>[8x]AMWHTHSEREKRVSNAVEFLL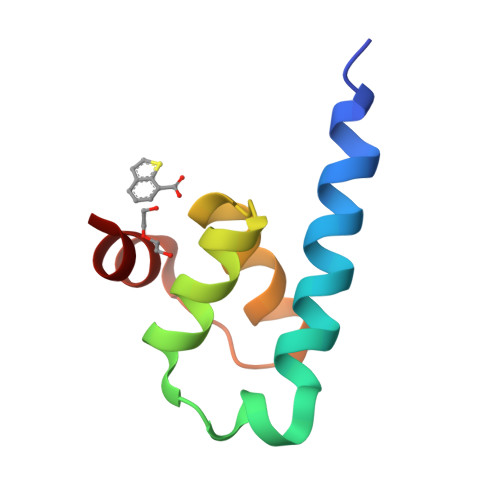DSRVRRTPTSSKVHFLKSKGLSAEEICEAFTKVGQPKTLNEIKRILS>MEYQIKYENGIANRGCLYRLKKVMDRAKAGEALNIAFLGGSITQGSLSSKPELCYAYHVYEWWKKTFPQADFTYINAGIGGTTSQFGVARAEADLLSKEPDFVIIEFSVNDDSTEHFMETYEGLVRKVYTSKTKPAVLLVHNVFYNNGANAQLMHGRIARHYNLPAVSMQSTIYPEVVAGRIENREITPDDLHPNDAGHALVASVITYFLDKVKTEDATEQSEPDYPAPLTKNTYEKSIRHQNSDENVVCHGFVADTSAQRDITDCFKHGWTASKKGDSITLDVEGCNISVQYRKSVKLPAPVAEIIVDGDAEHAVRLDANFDET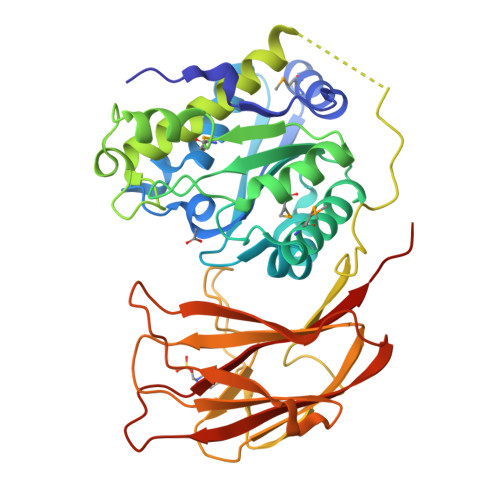WGDKLELDTILEHGENKVHKVEVRLTETHENDAVPFYLVSVIGSSEKAHHHHH[4x]> MSEMQGNKIVVDPITRIEGHLRIEVEVEGGKIKNAWSMSTLFRGLEMILKGRDPRDAQHFTQRACGVCTYVHALASVRAVDNCVGVKIPENATLMRNLTMGAQYMHDHLVHFYHLHALDWVNVANALNADPAKAARLANDLSPRKTTTESLKAVQAKVKALVESGQLGIFTNAYFLGGHPAYVLPAEVDLIATAHYLEALRVQVKAARAMAIFGAKNPHTQFTVVGGCTNYDSLRPERIAEFRKLY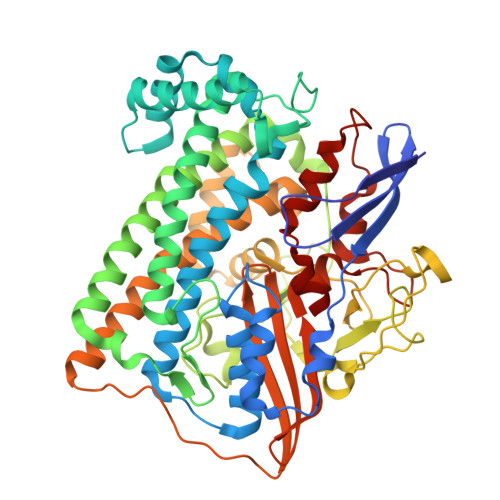KEVREFIEQVYITDLLAVAGFYKNWAGIGKTSNFLTCGEFPTDEYDLNSRYTPQGVIWGNDLSKVDDFNPDLIEEHVKYSWYEGADAHHPYKGVTKPKWTEFHGEDRYSWMKAPRYKGEAFEVGPLASVLVAYAKKHEPTVKAVDLVLKTLGVGPEALFSTLGRTAARGIQCLTAAQEVEVWLDKLEANVKAGKDDLYTDWQYPTESQGVGFVNAPRGMLSHWIVQRGGKIENFQLVVPSTWNLGPRCAEGKLSAVEQALIGTPIADPKRPVEILRTVHSYDPCIACGVH>[8x]MSELEKAMV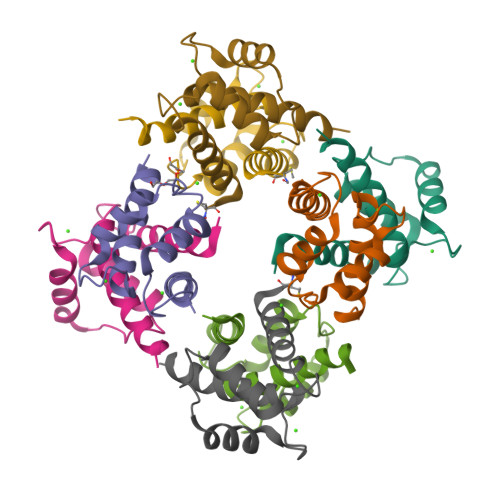ALIDVFHQYSGREGDKHKLKKSELKELINNELSHFLEEIKEQEVVDKVMETLDNDGDGECDFQEFMAFVAMVTTACHEFFEHE(2S)-HYDROXY(4-HYDROXYPHENYL)ETHANENITRILE | C8 H7 N O2 | 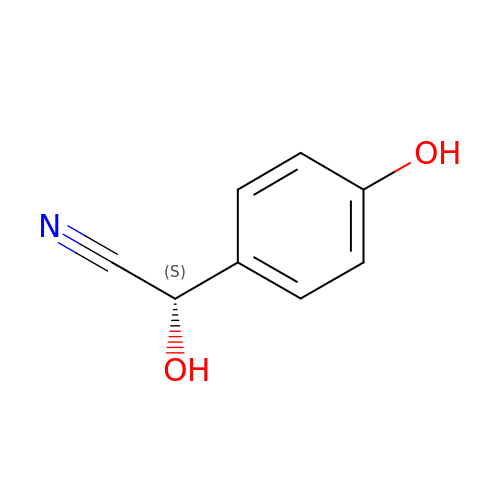HOOOPXDSCKBLFG-MRVPVSSYSA-N>SMMELRVGNRYRLGRKIGSGSFGDIYLGTDIAAGEEVAIKLECVKTK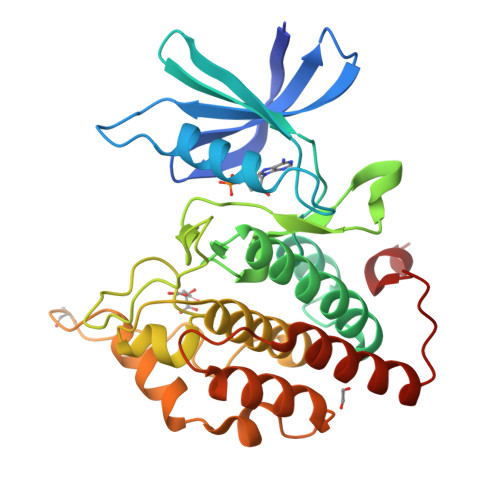HPQLHIESKIYKMMQGGVGIPTIRWCGAEGDYNVMVMELLGPSLEDLFNFCSRKFSLKTVLLLADQMISRIEYIHSKNFIHRDVKPDNFLMGLGKKGNLVYIIDFGLAKKYRDARTHQHIPYRENKNLTGTARYASINTHLGIEQSRRDDLESLGYVLMYFNLGSLPWQGLKAATKRQKYERISEKKMSTPIEVLCKGYPSEFATYLNFCRSLRFDDKPDYSYLRQLFRNLFHRQGFSYDYVFDWNMLK[2x]> GAPATVTEQGEDITSKKDRGVLKIVKRVGNGEETPMIGDKVYVHYKGKLSNGKKFDSSHDRNEPFVFSLGKGQVIKAWDIGVATMKKGEIAHLLIKPEYAYGSAGSLPKIPSNATLFFEIELLDFKGE

A typical example is the family of FK506‐binding proteins (FKBPs) that possess a highly conserved binding pocket but have diverged to perform diverse biological functions. The larger homolog FKBP51 is a regulator of glucocorticoid receptor (GR) signaling and has emerged as a potential target for depression, obesity‐induced diabetes and chronic pain. The most advanced FKBP51 ligands are compounds of the SAFit class (Selective Antagonists of FKBP51 by induced fit), which bind to a transient binding pocket unavailable to FKBP52 and are up to 10 000‐fold selective for FKBP51 over FKBP52. During a macrocyclization pilot study, we observed that many of these macrocyclic analogs have unanticipated and unprecedented preference for FKBP51 over FKBP12 and FKBP12.6.

As intended, the interactions of the pipecolate, the A‐ and B‐rings, as well as the cyclohexyl group with FKBP51 were completely conserved in comparison to previous FKBP51‐SAFit co‐crystal structures. Strikingly, we observed that the carbonyl group of 13 a, 13 d and 13 h displaced D68 and replaced it as a hydrogen bond acceptor for the ϵ‐hydroxy group of Y57. The rearrangement of the β3b strand is stabilized by an inward flip of H71, which partially replaces S70 and substitutes the former as a hydrogen bond donor for the backbone carbonyl of Y57. Intriguingly, H71 is replaced in FKBP12 and FKBP12.6 by an arginine (R40 in FKBP12/12.6 numbering), which can be expected to be less efficient in stabilizing the 13 a‐binding conformation, providing a molecular rationale for the discrimination vs. FKBP12/12.6 observed for the macrocycles. Representative macrocyclic compounds 13 c, 13 e and 13 h as well as SAFit1 and ‐2 all dose‐dependently competed with a fluorescent NanoBRET tracer inside cells. Compound 13 d as well as compounds 13 c, 13 e, 13 h and 13 i all inhibited IKKα phosphorylation, similar to SAFit1 and SAFit2 [4f]. For 13 c, 13 d and 13 h, the apparent maximal inhibition was already reached at the lowest tested concentration of 1 μm, possibly reflecting the higher affinities and/or improved cell permeability of 13 c, 13 d and 13 h compared to 13 e and 13 i.> QKLTVSHIEGYECQPIFLNVLEAIEPGVVCAGHDNNQPDSFAALLSSLNELGERQLVHVVKWAKALPGFRNLHVDDQMAVIQYSWMGLMVFAMGWRSFTNVNSRMLYFAPDLVFNEYRMHKSRMYSQCVRMRHLSQEFGWLQITPQEFLCMKALLLFSIIPVDGLKNQKFFDELRMNYIKELDRIIACKRKN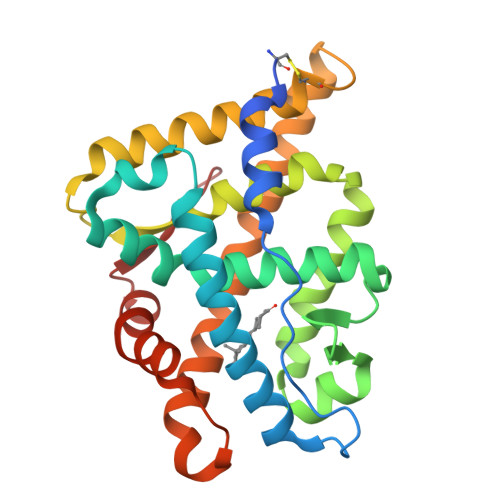PTSCSRRFYQLTKLLDSVQPIARELHQFTFDLLIKSHMVSVDFPEMMAEIISVQVPKILSGKVKPIYFHTQ Complementary DNA analyses revealed 22 distinct but similar peptides encoded by milk genes with homology to the lipocalin family of lipid-binding proteins, which are referred to as lipocalin-like milk proteins or Lili-Mip in this article. The data revealed glycosylated proteins that adopt a lipocalin fold, bind lipids and organize to form a tightly packed crystalline lattice. Lili-Mip serves as a complete nutrient by providing all of the essential amino acids, carbohydrates from the attached glycans, and lipids through chaperoning linoleic and oleic acids. After ingestion by the embryos, its increasing concentration in the midgut facilitates the crystallization of Lili-Mip.

Additionally, several crystals were solubilized and recrystallized in vitro. A third data set was collected from an in vitro-grown Lili-Mip crystal. The in vitro recrystallization of the solubilized Lili-Mip crystals, using only higher molecular-weight polyethylene glycol, demonstrated the high propensity of this protein for crystallization. In all cases, Lili-Mip crystallized in the triclinic P1 lattice, with one molecule per asymmetric unit and unit-cell parameters a = 32.28, b = 33.22, c = 40.18 Å, α = 99.5, β = 100.28, γ = 104.11°. Amino-acid sequence heterogeneity was observed in the structures determined from all three data sets.

> IAAILVANAKEPCPPENLQLPPRALVGKWYLRTTSPDIFKQVSNITEFYSAHGNDYYGTVTDYSPEYGLEAHRVNLTVSGSTLKFYMNDTHDYDSEYQILAVDKDYFIFYGHPPAAPSGLALIHYRQSCPKEDVIKRVKKNLKNVCLDYKYFGNDTSVPCHYVE>[2x]QAMVVKPLFPWDETLKFDHFSIILAPGALSESTPHEAGVIEHVVVISGEL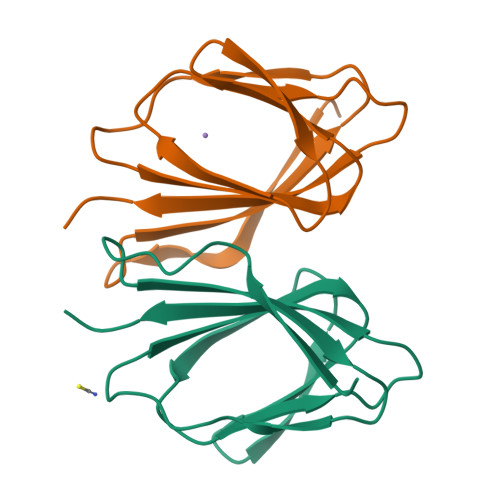EMKIDGEWRTLYPDQGVRFAGDKPHAYRNSSSRPVHFHSLIHYPR>[2x]MSLSVKVIVTDMDGTFLNDAKTYNQPRFMAQYQELKKRGIKFVVASNNQ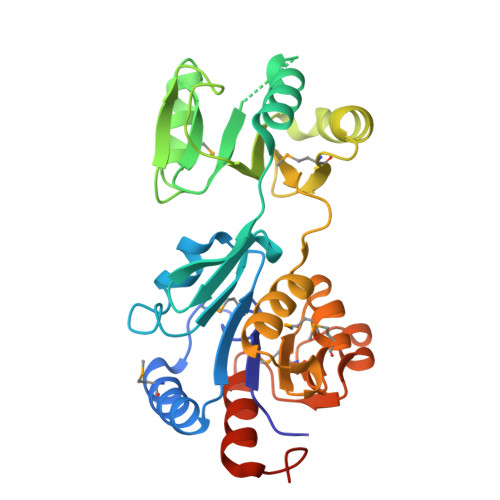YYQLISFFPELKDEISFVAENGALVYEHGKQLFHGELTRHESRIVIGELLKDKQLNFVACGLQSAYVSENAPEAFVALMAKHYHRLKPVKDYQEIDDVLFKFSLNLPDEQIPLVIDKLHVALDGIMKPVTSGFGFIDLIIPGLHKANGISRLLKRWDLSPQNVVAIGDSGNDAEMLKMARYSFAMGNAAENIKQIARYATDDNNHEGALNVIQAVLDNTSPFNSEGGSHHHHHH Volume-regulated anion channels (VRACs) are expressed widely in vertebrate cell types where they mediate the efflux of Cl- and organic solutes required for cell volume regulation. 8C-8A(IL125) consists of a 25-amino acid sequence unique to the first intracellular loop, IL1, of LRRC8A inserted into the corresponding region of LRRC8C. Like native VRAC/LRRC8 channels, 8C-8A(IL125) chimeras are activated strongly by cell swelling and low intracellular ionic strength. We demonstrate that the 8C-8A(IL125) chimeric channel is a large-pore seven-subunit heptamer, like homologous pannexin channels.

We obtained five distinct 3D classes for the 8C-8A(IL125) chimera. The 8C-8A(IL125) maps showed no apparent symmetric arrangement. Therefore, the final reconstructions were done without enforcing any symmetry and resulted in five structures with resolutions in the range of 3.4–4.0 Å (Figure 2—figure supplements 1 and 2). The most apparent difference between the structures is in the arrangement of the LRRDs. The arrangements of the LRRDs in the other three 3D classes exhibit diverse arrangements and subunit interactions. As a result, several different subunit interfaces exist between the neighboring LRRDs. The distances between the subunits forming the tight interfaces appear similar in all classes, whereas the distances between the subunits forming the loose interfaces are variable among different classes. The distinct arrangement of the loops formed by D50 and K51 is also observed in other classes. However, the number of subunits with K51 pointing toward the pores differs. For example, the class 2 structure has only one subunit with K51 pointing toward the pore, compared to two subunits in the class 1 structure. The groove created by the distinct K51 arrangement is located between the subunits that form one of the two loose interfaces in the class 2 structure, despite the presence of two loose interfaces.

>MIPVTEFRQFSEQQPAFRVLKPWWDVFTDYLSVAMLMIGVFGCTLQVMQDKIICLPKRVQPAQNHSSLSNVSQAVASTTPLPPPKPSPANPITVEMKGLKTDLDLQQYSFINQMCYERALHWYAKYFPYLVLIHTLVFMLCSNFWFKFPGSSSKIEHFISILGKCFDSPWTTRALSEVSGEDSDPKPAFSKMNGSMDKKSSTVSEDVEGSLVNSQSLKSIPEKFVVDKSTAGALDKKEGEQAKALFEKVKKFRLHVEEGDILYAMYVRQTVLKVIKFLIIIAYNSALVSKVQFTVDCNVDIQDMTGYKNFSCNHTMAHLFSKLSFCYLCFVSIYGLTCLYTLYWLFYRSLREYSFEYVRQETGIDDIPDVKNDFAFMLHMIDQYDPLYSKRFAVFLSEVSENKLKQLNLNNEWTPDKLRQKLQTNAHNRLELPLIMLSGLPDTVFEITELQSLKLEIIKNVMIPATIAQLDNLQELSLHQCSVKIHSAALSFLKENLKVLSVKFDDMRELPPWMYGLRNLEELYLVGSLSHDISRNVTLESLRDLKSLKILSIKSNVSKIPQAVVDVSSHLQKMCIHNDGTKLVMLNNLKKMTNLTELELVHCDLERIPHAVFSLLSLQELDLKENNLKSIEEIVSFQHLRKLTVLKLWHNSITYIPEHIKKLTSLERLSFSHNKIEVLPSHLFLCNKIRYLDLSYNDIRFIPPEIGVLQSLQYFSITCNVESLPDELYFCKKLKTLKIGKNSLSVLSPKIGNLLFLSYLDVKGNHFEILPPELGDCRALKRAGLVVEDALFETLPSDVREQMKTEENLYFQGAAAGDYKDDDDK[7x]2-oxo-4-propyl-2H-1-benzopyran-7-yl 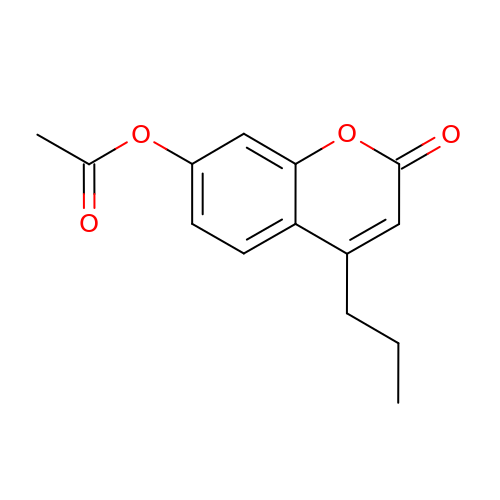acetate | C14 H14 O4 | LYHONYWOPDLTBH-UHFFFAOYSA-N[1-[1-(6-CARBAMOYL-CYCLOHEX-2-ENYLCARBAMOYL)-CYCLOHEXYLCARBAMOYL]-2-(4-PHOSPHONOOXY-PHENYL)- ETHYL]-CARBAMIC ACID 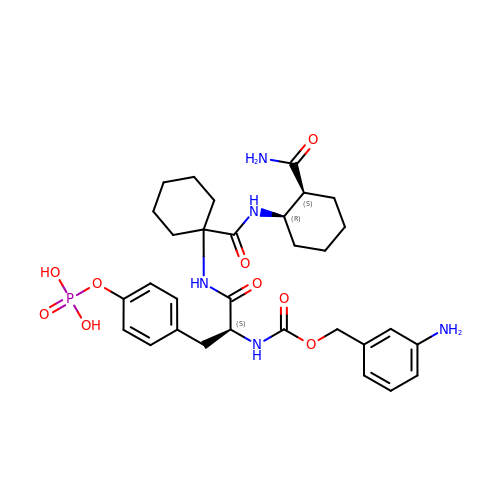3-AMINOBENZYLESTER | C31 H42 N5 O9 P | SLNOMHLVQNIGRT-NXCFDTQHSA-N>GAHMTRNGPGQTTGHPYYLRSFLVVLKTVLENEDDMLLFDEQEKGIVTKFYQLSATGQKLYVRLFQRKLSWIKMTKLEYEEIALDLTPVIEELTNAGFLQTESELQELSEVLELLSAPELKSLAKTFHLANPNGQKQQLVDAFLKLAKQRSVIGAVILKRAKALAGQSVRICKGPRAVFSRILLLFSLTDSMEDEDAACGGQGQLSTVLLVNLGRMEFPSYTINRKTHIFQDRDDLIRYAAATHMLSDISSAMANGNWEEAKELAQCAKRDWNRLKNHPSLRCHEDLPLFLRCFTVGWIYTRILSRFVEILQRLHMYEEAVRELESLLSQRIYCPDSRGRWWDRLALNLHQHLKRLEPTIKCITEGLADPEVRTGHRL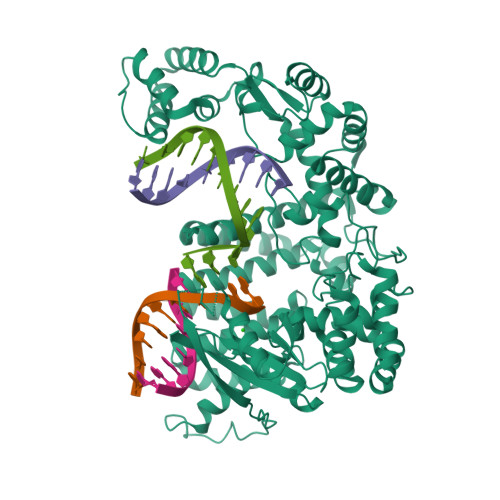SLYQRAVRLRESPSCKKFKHLFQQLPEMAVQDVKHVTITGRLCPQRGMCKSVFVMEAGEAADPTTVLCSVEELALAHYRRSGFDQGIHGEGSTFSTLYGLLLWDIIFMDGIPDVFRNACQAFPLDLCTDSFFTSRRPALEARLQLIHDAPEESLRAWVAATWHEQEGRVASLVSWDRFTSLQQAQDLVSCLGGPVLSGVCRHLAADFRHCRGGLPDLVVWNSQSRHFKLVEVKGPNDRLSHKQMIWLAELQKLGAEVEVCHVVAVGAKSQSLS[2x]> MNKKQNFYAAIIVAIFLCLQLSHGSSGVSFEKTPAIKIVGNKFFDSESGEQFFIKGIAYQLQRSEEELSNANGAFETSYIDALADPKICLRDIPFLKMLGVNTLRVYAIDPTKSHDICMEALSAEGMYVLLDLSEPDISINRENPSWDVHIFERYKSVIDAMSSFPNLLGYFAGNQVTNDHTNTFASPFVKAAIRDAKEYISHSNHRKIPVGYSTNDDAMTRDNLARYFVCGDVKADFYGINMYEWCGYSTYGTSGYRERTKEFEGYPIPVFFSEFGCNLVRPRPFTEVSALYGNKMSSVWSGGLAYMYFEEENEYGVVKINDNDGVDILPDFKNLKKEFAKADPKGITEEEYLTAKEPTEVESVECPHIAVGVWEANEKLPETPDRSKCACLDEILPCEIVPFGAESGKYEEYFSYLCSKVDCSD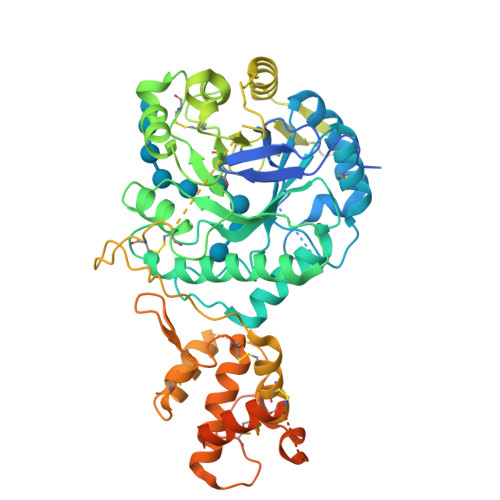ILANGKTGEYGEFSDCSVEQKLSLQLSKLYCKIGANDRHCPLNDKNVYFNLESLQPLTSESICKNVFDSIRDITYNHGDYSKSDPSRSKESLNVKYPSSEERENDGTIAFKTSGFVILLISMIAAGILL> ALTEGLGDELEEVIVEKTKQTVASISSGPKHTQKVPILTANETGATMPVLPSDSIETRTTYMHFNGSETDVECFLGRAACVHVTEIQNKDATGIDNHREAKLFNDWKINLSSLVQLRKKLELFTYVRFDSEYTILATASQPDSANYSSNLVVQAMYVPPGAPNPKEWDDYTWQSASNPSVFFKVGDTSRFSVPYVGLASAYNCFYDGYSHDDAETQYGITVLNHMGSMAFRIVNEHDEHKTLVKIRVYHRAKHVEAWIPRAPRALPYTSIGRTNYPKNTEPVIKKRKGDIKSY;> SPNVEACGYSDRVQQITLGNSTITTQEAANAVVCYAEWPEYLPDVDASDVNKTSKPDTSVCRFYTLDSKTWTTGSKGWCWKLPDALKDMGVFGQNMFFHSLGRSGYTVHVQCNATKFHSGCLLVVVIPEHQLASHEGGNVSVKYTFTHPGERGIDLSSANEVGGPVKDVIYNMNGTLLGNLLIFPHQFINLRTNNTATIVIPYIN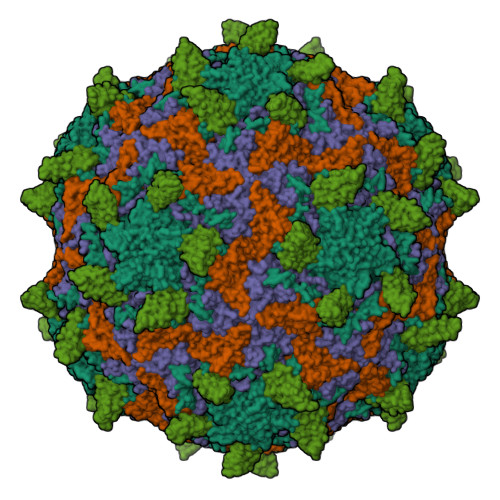SVPIDSMTRHNNVSLMVIPIAPLTVPTGATPSLPITVTIAPMCTEFSGIRSKSIVPQ;> GLPTTTLPGSGQFLTTDDRQSPSALPNYEPTPRIHIPGKVHNLLEIIQVDTLIPMNNTHTKDEVNSYLIPLNANRQNEQVFGTNLFIGDGVFKTTLLGEIVQYYTHWSGSLRFSLMYTGPALSSAKLILAYTPPGARGPQDRREAMLGTHVVWDIGLQSTIVMTIPWTSGVQFRYTDPDTYTSAGFLSCWYQTSLILPPETTGQVYLLSFISACPDFKLRLMKDTQTISQTVALTE;> GAQVSTQKSGSHENQNILTNGSNQTFTVINYYKDAASTSSAGQSLSMDPSKFTEPVKDLMLKGAPALN;> QTSVSPSKVILPRGGSVLVTCSTSCDQPKLLGIETPLPKKELLLPGNNRKVYELSNVQEDSQPMCYSNCPDGQSTAKTFLTVYWTPERVELAPLPSWQPVGKNLTLRCQVEGGAPRANLTVVLLRGEKELKREPAVGEPAEVTTTVLVRRDHHGANFSCRTELDLRPQGLELFENTSAPYQLQTFVLPATPPQLVSPRVLEVDTQGTVVCSLDGLFPVSEAQVHLALGDQRLNPTVTYGNDSFSAKASVSVTAEDEGTQRLTCAVILGNQSQETLQTVTIYSFPAPNVILTKPEVSEGTEVTVKCEAHPRAKVTLNGVPAQPLGPRAQLLLKATPEDNGRSFSCSATLEVAGQLIHKNQTRELRVLYGPRLDERDCPGNWTWPENSQQTPMCQAWGNPLPELKCLKDGTFPLPIGESVTVTRDLEGTYLCRARSTQGEVTRKVTVNVLSPRYE> MIPPPEKVRMNSVNFKNILQWEVPAFPKTQLTFTAQYESYRSFQDHCKRTASTQCDFSHLSKYGDYTVRVRAELADEHSEWVQVTFCPVEDTIIGPPEMQIESLAESLHLRFSAPQIENEPETWTLKNIYDSWAYRVQYWKQGTNEKFQVVSPYDSEVLRNLEPWTTYC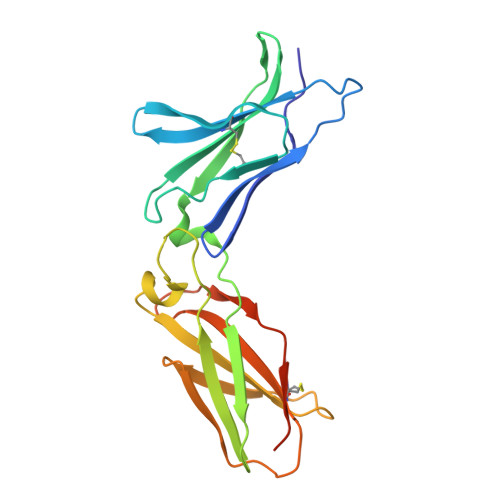IQVQGFLLDQQRTGEWSEPICERTGNDEITPSGGS The RoboDiff forms the core of the services offered on the ESRF beamline MASSIF-1 and, thus far, has been used to mount, characterize and collect diffraction data from over 20 000 samples since September 2014. In all three cases diffraction images were indexed and integrated using XDS and reduced using AIMLESS.

ARP/wARP was then run for automatic model building. Both models were completed manually using Coot interspersed with refinement with REFMAC5.

> TGTSTVGVGRGVLGDQKNINTTYSTYYYLQDNTRGDGIFTYDAKYRTTLPGSLWADADNQFFASYDAPAVDAHYYAGVTYDYYKNVHNRLSYDGNNAAIRSSVHYSQGYNNAFWNGSEMVYGDGDGQTFIPLSGGIDVVAHELTHAVTDYTAGLIYQNESGAINEAISDIFGTLVEFYANKNPDWEIGEDVYTPGISGDSLRSMSDPAKYGDPDHYSKRYTGTQDNGGVHINSGIINKAAYLISQGGTHYGVSVVGIGRDKLGKIFYRALTQYLTPTSNFSQLRAAAVQSATDLYGSTSQEVASVKQAFDAVGVK4-(3-chloro-5-cyanophenoxy)-3-[2-(2,4-dioxo-3,4-dihydropyrimidin-1(2H)-yl)ethoxy]phenyl sulfurofluoridate | C19 H13 Cl F N3 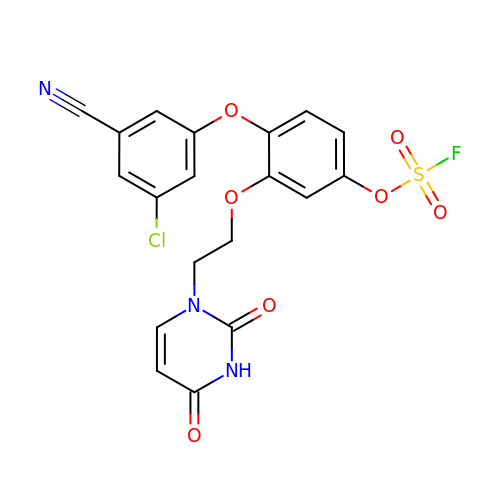O7 S | RUICQBSNQUGNNJ-UHFFFAOYSA-N>[3x]GDDHQGIIPLPPVENAFQEKYPDAKNPVFEIEGNYYVVDFNNGGSETTAWFTDQGIWMMEKIDISFAQLPAAVSTAFKQSFYSNWTVDDTYAINRLNMGIVYKIEAEQSNSEVDLYYSQYGNLIKAVDDEINNDAPIVIPKEVSNLMEITFANAELLDIQQNSLGYELDMIDNQIYKVAQLNKDYRWQSTTWAMSEQ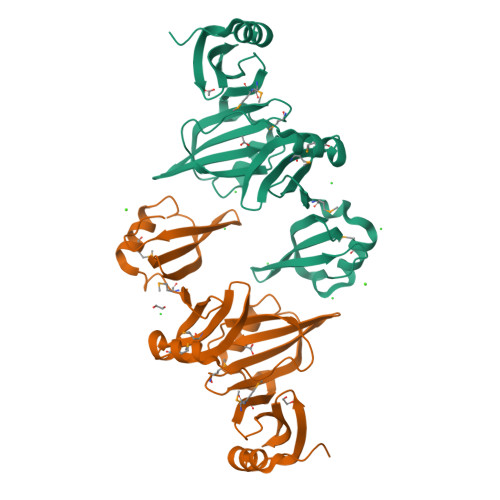EVPQIVMQGFESSAYASDKVQSIYTLLNANGTFYLFKVSHNGQDKTITFDVFGNIV The Type-IV restriction endonuclease (REase)ScoA3McrA (abbreviated as ScoMcrA hereafter) catalyzes multiple double strand cleavages 16–28 nucleotides (nt) away from the phosphorothioate linkage with the core sequence GPSGCC/GPSGCC. The DNA PT-dependent REase ScoMcrA distinguishes PT-DNA from normal DNA which differs only by one oxygen-to-sulfur swap, and presumably encodes a domain to specifically recognize sulfur on PT-DNA. Each ScoMcrA protomer consists of a head domain, an uncharacterized domain, a SRA-like domain, and an HNH domain. The uncharacterized domain binds specifically to PT-DNA whose sulfur atom is in the Rp but not in the Sp configuration, therefore we named it sulfur-binding domain (SBD).

Similar to the FL ScoMcrA protein, ScoMcrA‒SBD-SRA forms a dimer, with the SRA domain mediating dimerization but no association with PT-DNA. Although there are sulfur atoms in both strands of PT-DNA, which contain a palindromic GPSGCC core sequence, only one sulfur atom in PT-DNA is recognized by ScoMcrA-SBD in both structures. In support of these structural observations, both FL ScoMcrA and ScoMcrA-SBD interacted with hemi-PT-DNA, which has only one of the two DNA strands phosphorothioated, as shown in EMSA assays (lane 5 in Fig. 1a and Supplementary Fig. 5). By combining the structures of FL ScoMcrA and SBD-SRA in complex with PT-DNA, we obtained a model of FL ScoMcrA dimer recognition and cleavage of PT-DNA, which agrees well with our cleavage data. Our model suggests two ScoMcrA might not bind to two strands of one DNA at the same time.

> GSREAPKTFHRRVGDVRPARRAMGPALHRPVLLLWAIGQAVARAPRLQPWSTTRDAVAPLMEKYGQVEDGVDGVRYPFWALVRDDLWCVEQAEELTLTSRGRRPTLESLNAVDPSAGLREDDYNLLRSQPEAAASAAAGLIARYFHLLPAGLLEDFGLHELLAGRWPDALRPLLGETFKDRDAIWRAYGGQKMAGIGCLADGILSAFSDDKGPYADGRIPDTTWIAYVGDGLSGDQKLTDGNELMAEHQAVGRALRYWHKPFQGQWSFETWAVIVQRRLRWGLGEDKLPRREFLWVLAPVPSPERETWPPEVLEALEADTGELHDDTGDYRPSDLALTPGAPDGTESDDEAYRR PGNs are normally recognized, and/or hydrolyzed (amidases EC 3.5.1.28) in some cases, by a class of PRRs, termed peptidoglycan recognition proteins (PGRPs). The catalytic PGRPs possess the amidase activity that hydrolyzes the amide bond between the MurNAc and L-alanine moieties of PGN, via a coordinated Zn2+ ion. The full-length BbtPGRP3 consists of an N-terminal signal peptide (Met1−Ala18), followed by a CBD (Gln19−Tyr71) and a C-terminal PGRP domain (Thr90−Gly255), which are connected via an 18-residue linker from residues Ser72 to Gly89. All together, the modular evolution via gene horizontal transfer and domain shuffling results in a unique domain organization of BbtPGRP3, which has a higher amidase activity and a broader spectrum against invading bacteria.

The PGRP domain shows a typical PGN-binding domain scaffold, in which six β-strands (β4~9) compose a central β-sheet surrounded by five α-helices (α2~6) and a short 310 helix η1. The two disulfide bonds (Cys91-Cys214 and Cys128-Cys134) further stabilize the PGRP domain. Multiple-sequence alignment showed that BbtPGRP3 possess a highly conserved Gly-Tyr motif (Gly150-Tyr151) and an arginine residue Arg170, which are featured in the Group II PGRPs. Using HADDOCK server, we docked tracheal cytotoxin (TCT, GlcNAc-MurNAc(1,6-anhydro)-L-Ala-γ-D-Glu-meso-Dap-D-Ala) and muramyl pentapeptide (MPP, MurNAc-L-Ala-D-isoGln-L-Lys-D-Ala-D-Ala), which represent the DAP-type and Lys-type PGNs respectively, to the active-site valley of PGRP domain. The side-chain carboxylate of DAP forms a bidentate salt bridge with the guanidinium group of the conserved Arg170 docked TCT-complexed model, whereas residues Gly150 and Tyr151 interact with the side chain of L-Lys via van der Waals interactions in the MPP-complexed model. Moreover, structural comparison suggested that the complementary electropotential between DAP and Arg170 makes DAP-type PGN a favored substrate. Compared to the individual PGRP domain, fusion of the CBD resulted in an approximately 500% augmentation of activity towards S. aureus PGNs, compared to a 50% increase towards E. coli PGNs. It indicated that CBD contributes to the hydrolytic activity towards PGNs (especially the Lys-type) of the PGRP domain.

> MKSSHHHHHHENLYFQSNAQRWRSDGRCGPNYPAPDANPGECNPHAVDHCCSEWGWCGRETSHCTCSSCVDYSAGGGSSGGSTVVVSSSGTCPRIVSKSEWGSRATNYNVFLSLPVPKVVIHHSAGATCSTQSSCSLQVRNIQNYHMDGRGYSDIGYNFLVGNDGNVYEGRGWDRRGAHALNVNTESIGICFMGDFTSQKPTASAIAAAKSLISCGVSLGKIRSGYSLYGHRDVGSTACPGNLLYDDIKSWGRYVG> MSGIGALFRPLPRMGPRLPFELPAPPRPHLPMPAPRPLPRPAPGALTLSRDRTREAERDCSKSQGRDKDCVECPPSRGEMAIANNGKGHSMSDLSARYQQWVTNFPFPHEWFWSGTWWDGFDEPRCTLLEAKANYAFLFVPLLGVPRPWARAKVKSDLLQKAEVHSDKARPTPPVFVEWHFLQRIVYEYCAAEYLRMGLANLKAFWNPMPGTDEHDDYQETRAKEQEEMKRFCEENPGYCA;> MTDAKAFRRYIFELYFDPARLLELDDDQHLQRIERFLDALAPLHPVLENWYLCGDSLRDALSHNVTEHRQDLAKALSRDRRTRAVELVLWNGEEDPLKGGLSLDYEASGRAVSSRLQLEDAGSLLQVFDAPASSFVAIFLAVL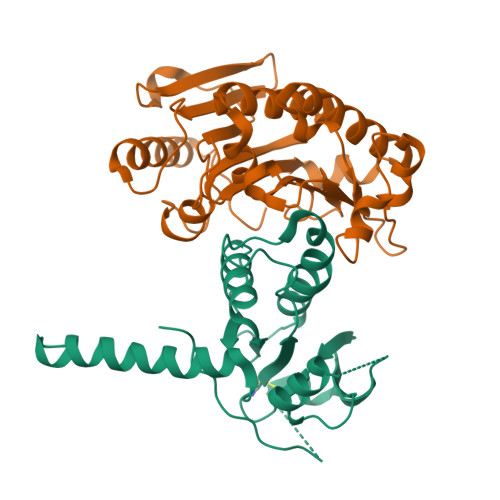EIWPETTWGMLAPHAYFVHQRTFPDRRSIGWIGFCPHPLRATDFPAATELVDIPGRGTLLLNGREPMDETRREHFERVGEADIKLMELGYLPPLRG> SVLRPQLTFEHPVDNSPTPFRPVYYDEKGVRHVGEPGVHPFAERIKAVSVPSEQLLLKTETPYLSLVTCPLTFVDTVEDLEALVAVLLNETEIAVDLEHHDFYSYQGFTCLMQISTRTQDFIVDCLKVRANMYLMAPVFLQPNIVKVFHGAREDVRWLQKDFGLYIVNLFDTSIALQNLHMPHSLAFAVDHFCQVKLNKKYQTADWRVRPIPAEMVSYAQQDTHFLLYVYDRLKQLLLNCEARASVGNMLLHVFQESRLLSLERYEKPHLDPDVTYKQALGRSLGGLSSSQLQVAREIFNWRDMAAREADDSPSAVMHISSVLSIATKLPTSANEVLKCCSPVSVAVRTNVMKLLQIVKDAIGSALEHHHHHH

The exosome is a 3′–5′ exoribonuclease complex that plays a central role in numerous pathways related to RNA processing and degradation, both in the nucleus and in the cytoplasm. The eleventh exosome subunit, RRP6, is a member of the DEDD superfamily (DEDD-Y subgroup) of divalent metal dependent exonucleases. Rrp6 is composed of an N-terminal PMCN2NT domain which was shown to interact with a cofactor Rrp47, the EXO domain containing the catalytic active site, an HRDC (helicase and RNAseD C-terminal) domain, and a C-terminal region responsible for the interaction with the exosome. The EXO domain consists of a classical α/β fold composed by a six-stranded β-sheet flanked by α-helices and the HRDC domain is constituted of six α-helices.

The electron density map revealed the presence of a disulfide bond between the residues C496 and C515, linking α-helix 3 and the end of α-helix 4 of the HRDC domain. In order to study the effect of the disulfide bond disruption on the protein structure and activity, site directed mutations were introduced in the cysteine residues generating the variants TbRRP6CAT-C496S and TbRRP6CAT-C595S. Crystallization trials were performed and crystals suitable for X-ray diffraction experiments were obtained for the mutant TbRRP6CAT-C496S. A complete data set was collected and the TbRRP6CAT-C496S structure was refined at 2.15 Å resolution to final Rfactor/Rfree of 17%/22%. Similarly to TbRRP6CAT the residues 416 to 423 could not be modeled. Superposition of TbRRP6CAT and the mutant TbRRP6CAT-C496S structures resulted in an RMSD of 0.51 Å for 352 C-alpha atoms aligned. The structural changes resulted from the disulfide bond disruption are restricted to one of the helices involved in the SS bond. In the oxidized protein, the short turn that follows helix 4 moves away from helix 3 for the SS bond formation. On the other hand, the mutants C496S and C595S showed activity comparable with the native protein, indicating that the disruption of the SS bond in the HRDC domain does not affect TbRRP6 degradation of non-structured substrates in vitro. The mutants TbRRP6CAT-C496S and TbRRP6CAT-C595S, lacking the SS bond, were also assayed against double-stranded RNA and showed activity comparable with the constructs with native cysteine residues.N-[4-[(2,4-DIAMINOFURO[2,3D]PYRIMIDIN-5-YL)METHYL]METHYLAMINO]-BENZOYL]-L-GLUTAMATE 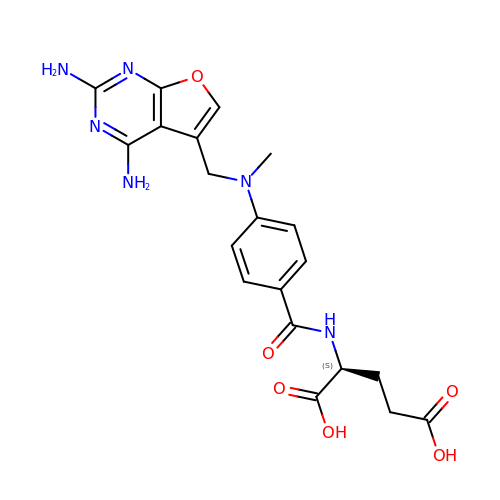| C20 H22 N6 O6 | WXINNGCGSCFUCR-ZDUSSCGKSA-N>HEVVKFMDVYQRSYCHPIETLVDIFQEYPDEIEYIFKPSCVPLMRCGGCCNDEGLECVPTEESNITMQIMRIKPHQGQHIGEMSFLQHNKCECRPKKD[2x];>[2x]GRPFVEMYSEIPEIIHMTEGRELVIPCRVTSPNITVTLKKFPLDTLIPDGKRIIWDSRKGFIISNATYKEIGLLTCEATVNGHLYKT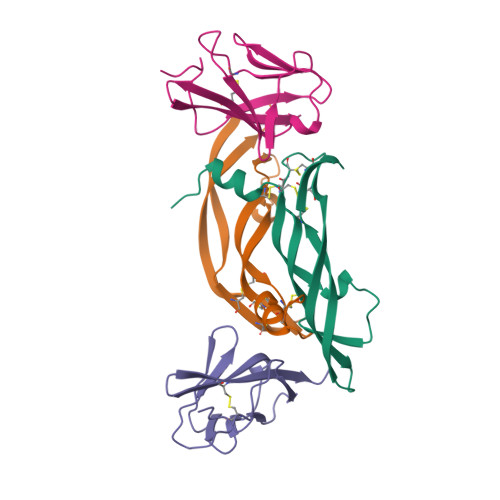NYLTHRQT>MELVVKSVAAASVKTATLVIPVGENRKLGAVAKAVDLASEGAISAVLKRGDLAGKPGQTLLLQNLQGLKAERVLLVGSGKDEALGDRTWRKLVASVAGVLKGLNGADAVLALDDVAVNNRDAHYGKYRLLAETLLDGEYVFDRFKSQKVEPRALKKVTLLADKAGQAEVERAVKHASAIATGMAFTRDLGNLPPNLCHPSFLAEQAKELGKAHKALKVEVLDEKKIKDLGMGAFYAVGQGSDQPPRLIVLNYQGGKKADKPFVLVGKGITFDTGGISLKPGAGMDEMKYDMCGAASVFGTLRAVLELQLPVNLVCLLACAENMPSGGATRPGDIVTTMSGQTVEILNTDAEGRLVLCDTLTYAERFKPQAVIDIATLTGACIVALGSHTTGLMGNNDDLVGQLLDAGKRADDRAWQLPLFDE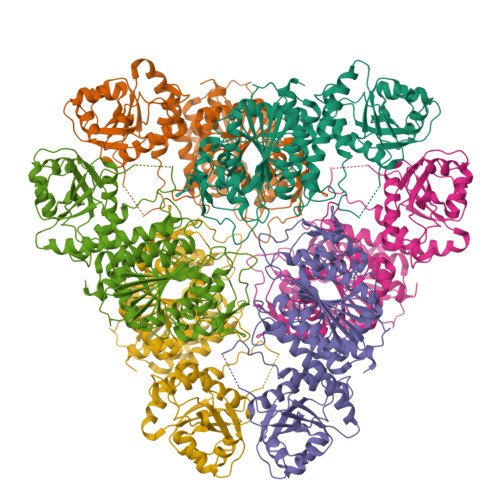YQEQLDSPFADMGNIGGPKAGTITAGCFLSRFAKAYNWAHMDIAGTAWISGGKDKGATGRPVPLLTQYLLDRAGA[2x]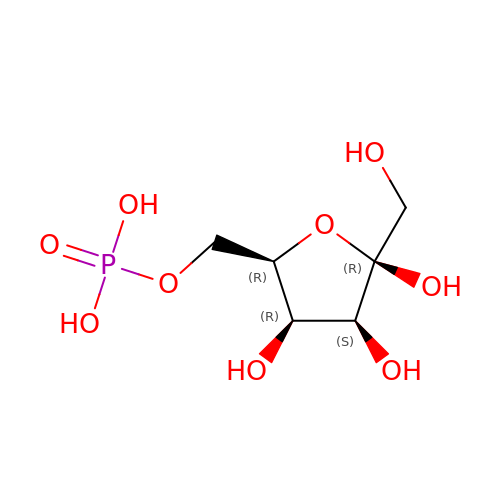6-O-phosphono-beta-D-tagatofuranose | C6 H13 O9 P | BGWGXPAPYGQALX-DPYQTVNSSA-N>[2x]GPGMAVKQLIVLKFKDEITEAQKEEFFKTYVNLVNIIPAMKDVYW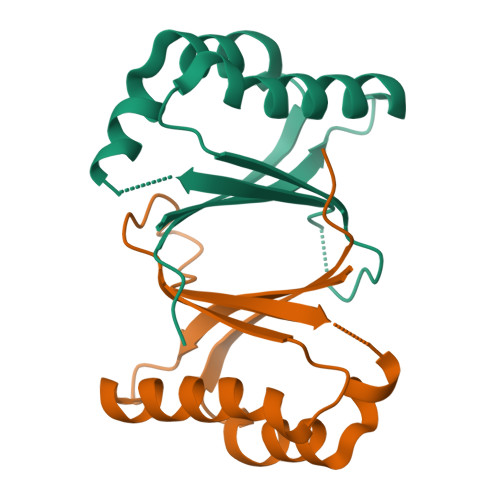GKDVTQKNKEEGYTHIVEVTFESVETIQDYIIHPAHVGFGDVYRSFWEKLLIFDYTPRK>GUCAUUCUAUUCUAUCGGCUAAGGAUGAAAGUCUA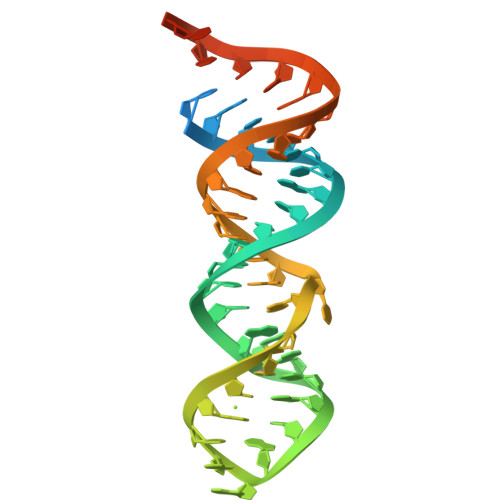UGCCGAUUCUAUUCUAUGGC[2x]The HIV-1 Trans-Activation Response element (TAR) RNA, located at both ends of its RNA genome, is one of the most conserved RNA structural elements in retroviruses. It assumes multiple, dynamic conformations to carry out critical functions in several stages of the HIV-1 life cycle, including reverse transcription, proviral transcription, genome dimerization and packaging, viral translation, and immune suppression, etc. Here, we report crystal structures of the full-length HIV-1 TAR which reveal substantial conformational mobility in its three conserved bulges and in its lower stem, which coordinately maintain the structural fluidity of the entire RNA. We find that TAR RNA is a robust inhibitor of PKR, and primarily uses its lower stem to capture and sequester PKR monomers, preventing their dimerization and activation.

To visualize the complete HIV-1 TAR structure and particularly the PKR-binding lower stem, we crystalized the 57-nt RNA by substituting the UGGG portion of the distal hexaloop with a GAAA tetraloop. In our full-length TAR structures, A17 is stably flipped out, allowing its two flanking stems to coaxially stack with and stabilize each other. While the unpaired A17 (or A16) residue located in the mid-section is stably bulged out, the other unpaired residue, C5, located near the termini, assumed three distinct conformations among the three structures. In TAR-Ia, C5 flips away from the termini and binds in the major groove, forming a base triple with the C9-G52 pair. In TAR-Ib, C5 flips towards the termini and binds the minor groove, forming an inclined base triple with the G3-C57 pair. A comparative analysis of the crystal structures of full-length TAR revealed that the C5 bulge can sample multiple locations, conformations, and contacts. Remarkably, the wider, axially compressed helix of TAR overlays nearly perfectly with the coaxially stacked apical stem and tetrastem portions of the Adenovirus VA-I RNA termed mini-VA, which is necessary and sufficient to inhibit PKR. Therefore, different viruses seem to have converged on a common RNA-based strategy to suppress PKR — by using short (24–28 bp), imperfect dsRNA segments to sequester PKR monomers.

>[2x]GGUCUCUCUGGUUAGACCAGAUCUGAGCCGAAAAGCUCUCUGGCUAACUAGGGAACC>[2x]NLLQFRKMIKCTIPGIEPLLAFSNYGCYCGK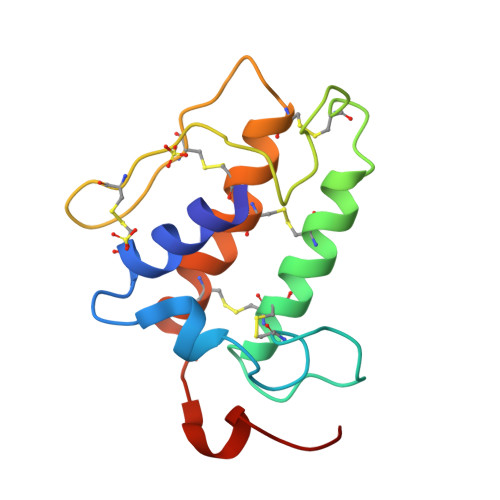GGSGTPVDELDRCCQTHDYCYDKAKIHPECRGILSGPSFNTYAYDCTDGKLTCNDQKDKCKLFICNCDRTAAMCFAKAPYKEENNRIDAS2-[(1S)-1-methylpropyl]-4,5-dihydro-1,3-thiazole | C7 H13 N S | 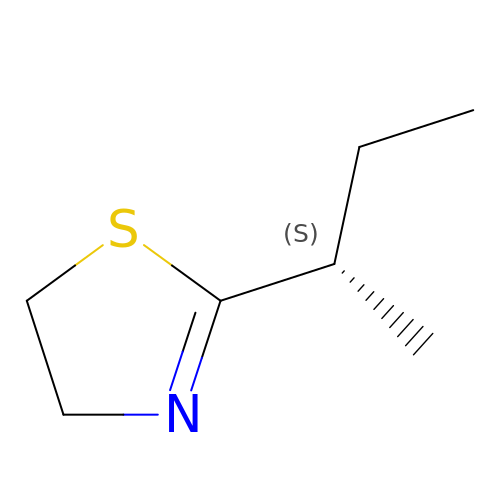SAWWKXMIPYUIBW-LURJTMIESA-N>GMKSQWECFLQNLGVWEGSFSNFSPEGTLLNDTSSRLCLEGLNNNQTVRLTLSRSGKDDVIREFRSVGGGLLFFENGSFSEGLIQLGPFSEFGGELAFVHENRRLRLVQLFDRNGHLNGLTLIREHLAGTPVAERPLLQINDLLGEWRGQAVTIYRDLRPPDIYSTT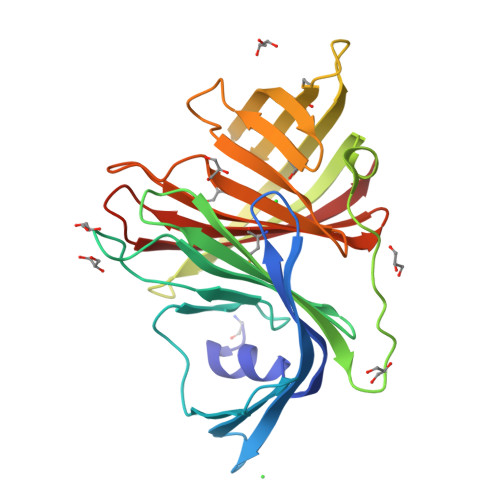LKIQLDDAGRLMQSTSFGERTITSTATIKGSIVLFDQDPEKQVQVLLLPDGASATSPLKVQLRQPLFLEAGWLIQSDLRQRMIRSYNDKGEWVSLTLVTEERV[2x]>[2x]MHHHHHHVMIMKAFISENVRGIYAFDENGNLIEKRYFTDKPEKVLDQLLKGEITKDLEELLNSLKEKGYDEFVFEHPELSRRAKELGFSATTEFPNIAGERLRSNPEEFLGENWFEEYYKVGVALTRMRIQEQSGARDKMVIQAIEALDDVDKVINLLVARLREWYSLHFPELDELLPKHPQYVAFVKTVGHRDNINEEVLRELGLSEEKIKKILEAKEKTMGAWMDQTDIEVVRQLAEEIDRLYQLRKKLEDYIDRAMDDVAPNLKALVGAKLAARLISLAGGLRELAMMPSSTIQVLGAEKALFRHLRTGAKPP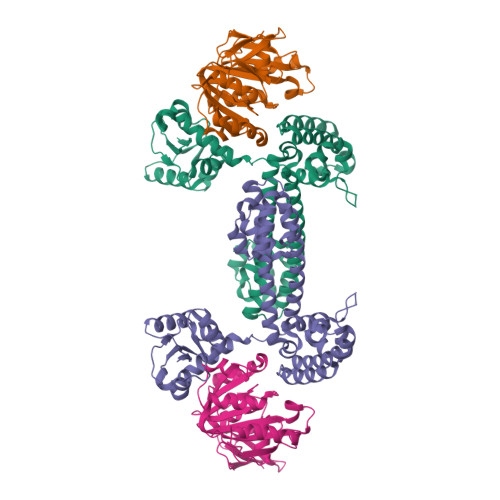KHGVIYQYPAINRSPWWQRGKIARALAGKLAIAARVDYFSGEYIAEELKKELEARIREIK;>[2x]MHHHHHHMVEVKKHKFPGVYVVIDDDGSEKIATKNLVPGQRVYGERVIKWEGEEYRIWNPHRSKLGAAIVNGLKNFPIKPGKSVLYLGIASGTTASHVSDIVGWEGKIYGIEFSPRVLRELVPIVEERRNIIPILGDATKPEEYRALVTKVDVIFEDVAQPTQAKILIDNAKAYLKRGGYGMIAVKSRSIDVTKEPEQVFKEVERELSEYFEVIERLNLEPYEKDHALFVVRKP> GGKSEKLQEHLVAEQTSTFTEKEVYSSDKLIIKQVSPHTYVHVSFLDTDTFGKVACNGMIVISDGEAVVFDTPSTSNETSELLSFLEEEKLQVNAVVATHFHLDCLGGLEAFHARNIPSYAFKNT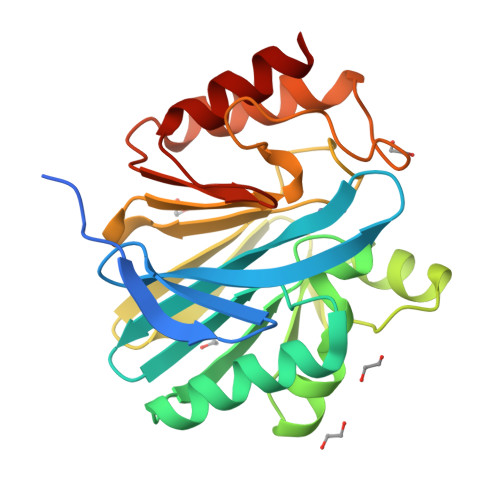LSLASQHDFPQPQKGFSDELTLKVGTKAVFVHYFGEGHTQDNVIGYFPDDQVLFGGCLIKANGAGKGNLEDANVEAWPVTVNKISTAYPNLRLVIPGHGNWGDKTLLHYTETLFK>[2x]MDRRKFIKTSLFSALGFSVGGLSLLSCGGGGTTGSSSGQGSGTLSKQSLNIPGYSLFSDGQRVSITAKWTTLEVIPGKSTDMLVYEIDNEYNPVIFLRKGQTFSADFVNNSGEDSIIHWHGFRAPWKSDGHPYYAVKDGETYSYPDFTIIDRSGTYFY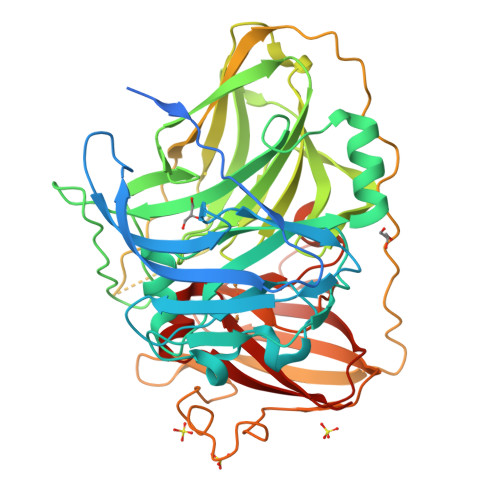HPHPHGRTGYQVYYGLAGMIIIEDEDEDNLKQALDLEYGVTDIPLIIQDKTFDSSGQLVYNPMGHMGFWGDTILVNLTPNPYMDVERKIYRFRILNGSNARPYRLALLRGNQRMRFWVIGVEGGLLDTPKEVNEILVAPGERIDILVDFRDASVNDVIKLYNFPHNLIGMGMIGMRMGMGMERGMGMGNGMNMDMGMADNSEFEVMEFRVTKDSAYDKSIPQRLSEVTPINTDGAQVQRITLGMRRMVFTINGETWEDGYANPQDINNPKVLFEQNNGDVVILEYVNNTGTYHPMHIHGFQFQVLERSLGPLGATDLGWKDTVIVAPMETVRIAVDMSHPYNEHQIYLLHCHILEHHDEGMMVNYRVNA>[2x]MGSSHHHHHHSSGRENLYFQGMIYQPDENRYHTMEYRRCGRSGVKLPAISLGLWHNFGDTTRVENSRALLQRAFDLGITHFDLANNYGPPPGSAECNFGRILQEDFLPWRDELIISTKAGYTMWDGPYGDWGSRKYLIASLDQSLKRMGLEYVDIFYHHRPDPETPLKETMKALDHLVRHGKALYVGISNYPADLARQAIDILE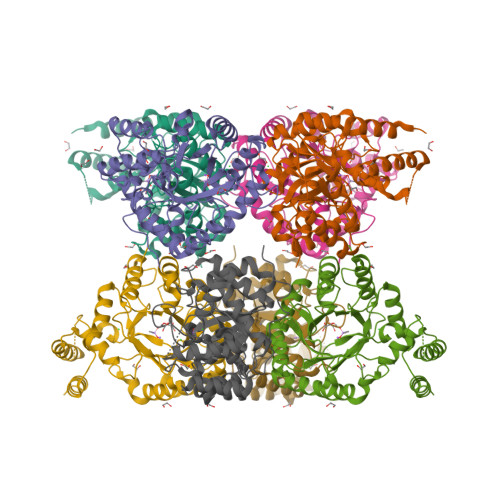DLGTPCLIHQPKYSLFERWVEDGLLALLQEKGVGSIAFSPLAGGQLTDRYLNGIPEDSRAASGSRFLKPEQITADKLEKVRRLNELAARRGQKLSQMALAWVLRNDNVTSVLIGASKPSQIEDAVGMLANRRFSAAECAEIDAILEGRF>GAMADPSEKETNYVENLLTQLENELNEDNLPEDINTLLRKCSLNLVTVVSLPDMDVKPLLATIKRFLTSNVSYDSLNYDYLLDVVDKLVPMADFDDVLEVYSAEDLVKALRSEIDPLKVAACRVIENSQPKGLFATSNIIDILLDILFDEKVENDKLITAIEKALERLSTDELIRRRLFDNNLPYLVSVKGRMETVSFVRLIDFLTIEFQFISGPEFKDIIFCFTKEEILKSVEDILVFIELVNYYTKFLLEIRNQDKYWALRHVKKILPVFAQLFEDTENYPDVRAFSTNCLLQLFAEVSRIEEDEYSLFKTMDKDSLKIGSEAKLITEWLELINPQYLVKYHKDVVENYFHVSGYSIGMLRNLSADEECFNAIRNKFSAEIVLRLPYLEQMQVVETLTRYEYTSKFLLNEMPKVMGSLIGDGSAGAIIDLETVHYRNSALRNLLDKGEEKLSVWYEPLLREY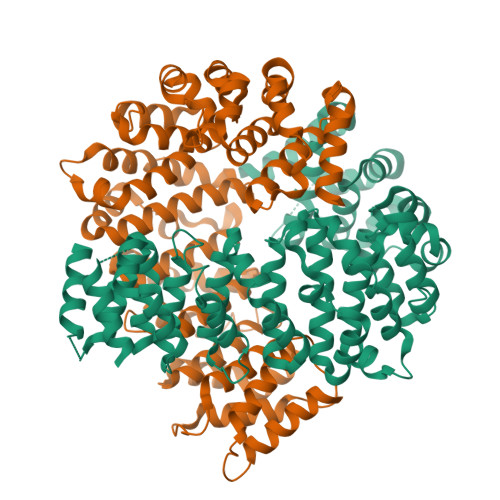SKAVNGKNYSTGSETKIADCR[2x]> NHASAPMTRA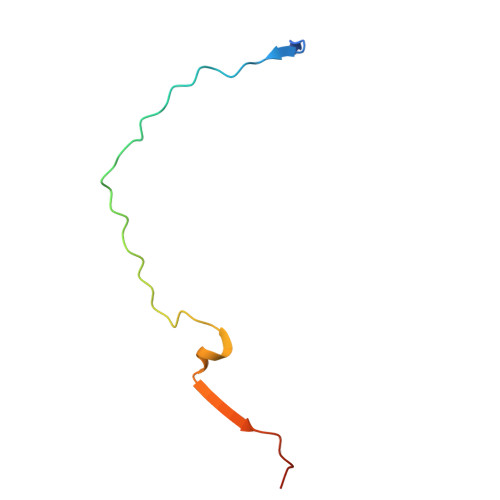PAPEYVPETPHHSDWQRPSFHFEGKGAAGGHSATRHASAPATRPQPVE>MAAGVAAWLPFARAAAIGWMPVASGPMPAPPRQERKRTQDALIVLNVSGTRFQTWQDTLERYPDTLLGSSERDFFYHPETQQYFFDRDPDIFRHILNFYRTGKLHYPRHECISAYDEELAFFGLIPEIIGDCCYEEYKDRRRENAERLQDDADTDTAGESALPTMTARQRVWRAFENPHTSTMALVFYYVTGFFIAVSVIANVVETVPCGSSPGHIKELPCGERYA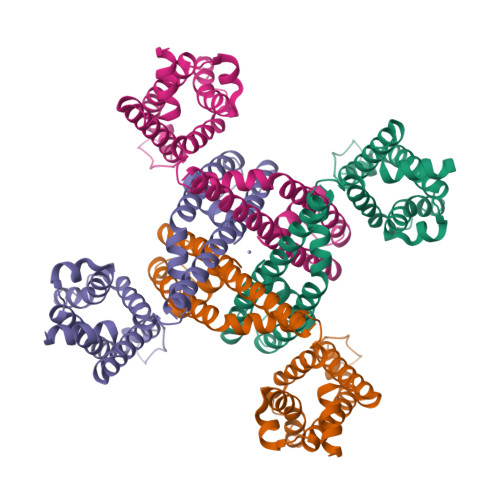VAFFCLDTACVMIFTVEYLLRLAAAPSRYRFVRSVMSIIDVVAILPYYIGLVMTDNEDVSGAFVTLRVFRVFRIFKFSRHSQGLRILGYTLKSCASELGFLLFSLTMAIIIFATVMFYAEKGSSASKFTSIPAAFWYTIVTMTTLGYGDMVPKTIAGKIFGSICSLSGVLVIALPVPVICSNFSRIYHQNQRADKRRAQKKARLARIRAAKSGSANAYMQSKRNGLLSNQLQSSEDEQAFVSKSGSSFETQHHHLLHCLEKTTNHEFVDEQVFEESCMEVATVNRPSSHSPSLSSQQG[4x]>[2x]MGSDKIHHHHHHMMWEQFKKEKLRGYLEAKNQRKVDFDIVEL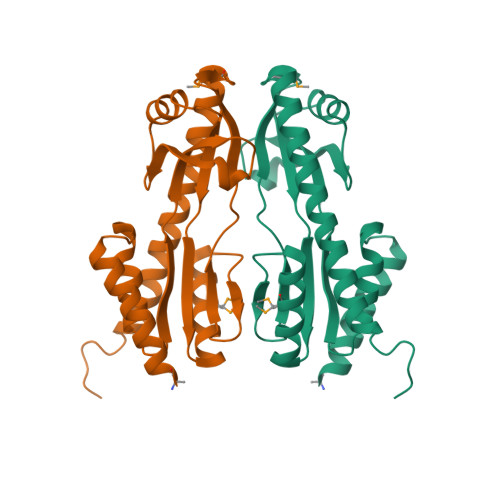LDLINSFDDFVTLSSCSGRIAVVDLEKPGDKASSLFLGKWHEGVEVSEVAEAALRSRKVAWLIQYPPIIHVACRNIGAAKLLMNAANTAGFRRSGVISLSNYVVEIASLERIELPVAEKGLMLVDDAYLSYVVRWANEKLLKGKEKLGRLQEALESLQRENAYCSD>MDFLSNFLTDFVGQLQSPTLAFLIGGMVIAALGTQLVIPEAISTIIVFMLLTKIGLTGGMAIRNSNLTEMLLPVAFSVILGILIVFIARFTLAKLPNVRTVDALATGGLFGAVSGSTMAAALTTLEESKISYEAWAGALYPFMDIPALVTAIVVANIYLNKRKRKSAAASIEESFSKQPVAAGDYGDQTDYPRTRQEYLSQQEPEDNRVKIWPIIEESLQGPALSAMLLGLALGIFTKPESVYEGFYDPLFRGLLSILMLIMGMEAWSRIGELRKVAQWYVVYSLIAPIVHGFIAFGLGMIAHYATGFSLGGVVVLAVIAASSSDISGPPTLRAGIPSANPSAYIGSSTAIGTPIAIGVC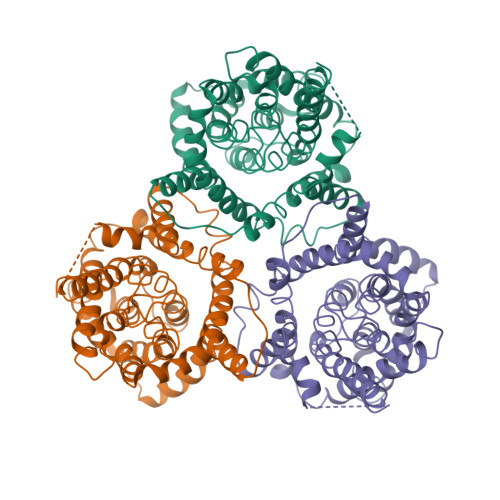IPLFIGLAQTLGAG[3x]> CLAVPGKVIEVNGPVAVVDFGGVKREVRLDLMPDTKPGDWVIVHTGFAIEKLDEKKAMEILEAWAEVEKAMEGF;> MEEPFEAYRSREVAMKLVEKIREEAKTLDGE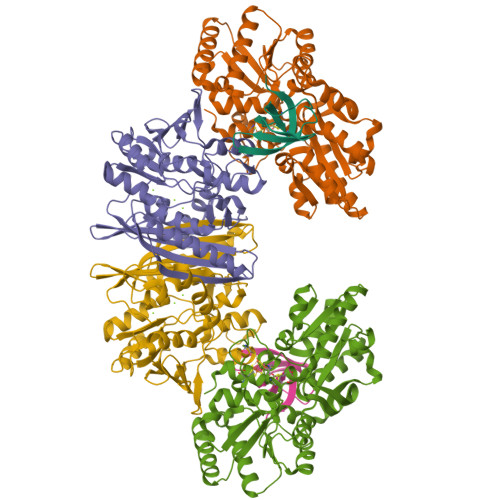IRIMHVCGTHEDTVTRHGIRSLLPENVKVVSGPGCPVCITPVEDIVAMQLIMRKAREEGEEIILTTFGDMYKIPTPMGSFADLKSEGFDVRIVYGIFDTYRIAKENPDKTVVHFSPGFETTTAPAAGMLNVAAQEELENFKIYSVHRLTPPAVEVLLKQGTVFQGLIAPGHVSTIIGVKGWEYLTEKYGIPQVVAGFEPNDVLMAILMLIRMYKEGEARIINEYERAVKYEGNVVAQKMIDKFFEVVDAKWRALGVFPKSGLELRKEWKDFEIRSFYKVEVPKNLPDLEKGCRCGAVLRGLALPTDCPLFGKTCTPRHPVGPCMVSYEGTCQIFYKYGVLF;> MGEKIKLEHGAGGEIMEELLRDVILKTLTLKSAGGIGLDALDDGATIPFGDKHIVFTIDGHTVKPLFFPGGDIGRLAVSGTVNDLAVMGAEPIALANSMIIGEGLDMEVLKRVLKSMDETAREVPVPIVTGDTKVVEDKIEMFVITAGIGIAEHPVSDAGAKVGDAVLVSGTIGDHGIALMSHREGIAFETELKSDVAPIWDVVKAVAETIGWENIHAMKDPTRAGLSNALNEIARKSNVGILVREADIPIRPEVRAASEMLGISPYDVANEGKVVMVVAREYAEEALEAMRKTEKGRNAAIIGEVIADYRGKVLLETGIGGKRFMEPPEGDPVPRIC T-STAR is a tissue-specific STAR protein mainly expressed in the testis and brain3426, and regulates the alternative splicing of CD44, Tra2β, Tau, VGEF and Neurexin pre-mRNAs262728. STAR proteins are defined by the presence of a highly conserved RNA-binding domain, the STAR domain, also responsible for homodimerization, and composed of a central KH (K homology) domain flanked by two highly conserved regions, QUA1 and QUA2. Here, we have determined the X-ray structures of the T-STAR KH domain in its free state, and in complex with AAAUAA; KH-QUA2 in complex with AAUAAU; QUA1-KH in complex with UAAU; and the full STAR domain in complex with AUUAAA. Taken together, our data reveal a unique mode of RNA recognition and dimerization by the STAR proteins Sam68 and T-STAR that is crucial for their function in alternative splicing.

All our structures of T-STAR in complex with RNA display a very similar mode of RNA recognition, and show that the KH domain specifically recognizes three nucleotides with the sequences U1A2A3 or A1A2A3 as illustrated for the structure of T-STAR KH-AAAUAA where one KH domain binds the 5′-AAA and another KH binds the 3′-UAA moieties of the RNA. The base of the nucleotide A3 is specifically recognized through intermolecular hydrogen bonds with the backbone atoms of I97 in β-strand 2 mimicking a Watson-Crick base pair. The base of the nucleotide A2 is specifically recognized through an intermolecular hydrogen bond to N71 side chain. Additional nucleotides located 5′ or 3′ of the (A/U)AA motif are visible in our structures but do not make specific contacts to the protein, suggesting that only the (A/U)AA motif is specifically recognized by T-STAR. Strikingly, no electron density could be observed for the QUA2 region of T-STAR in all our data sets, suggesting that the QUA2 region does not adopt a well-defined orientation. Interestingly, the presence of the QUA2 region in the STAR domains increases the radius of gyration and maximal dimensions both in the absence and presence of RNA. This is consistent with the QUA2 domain being flexibly attached to the QUA1-KH domain dimer, and may explain that no electron density is observed for the QUA2 domain in the crystal structures of the T-STAR STAR and KH-QUA2 domains. The absence of electron density for the QUA2 domain in our X-ray data sets suggests that the QUA2 domain of T-STAR does not contribute to RNA binding. Altogether, our data demonstrate that the QUA2 regions of Sam68 and T-STAR are not involved in RNA binding, in contrast to the other members of the STAR family SF1, QKI and GLD-1.

>GAINKNMKLGQKVLIPVKQFPKFNFVGKLLGPRGNSLKRLQEETLTKMSILGKGSMRDKAKEEELRKSGEAKYFHLNDDLHVLIEVFAPPAEAYARMGHALEEIKKFLIPDYNDEIRQAQLQELTYLNGGSENADV[2x]>[3x]SVVIVGKISFCPKDVLGHGAEGTIVYRGMFDNRDVAVKRILPECFSFADREVQLLRESDEHPNVIRYFCTEKDRQFQYIAIELCAATLQEYVEQKDFAHLGLEPITLLQQTTSGLAHLHSLNIVHRDLKPHNILISMPNAHG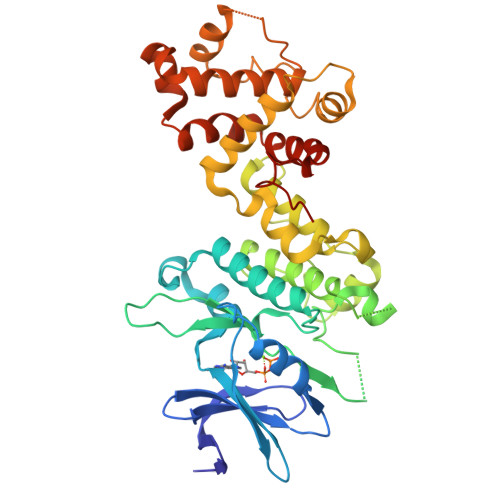KIKAMISDFGLCKKLAVGRHSFSRRSGVPGTEGWIAPEMLSEDCKENPTYTVDIFSAGCVFYYVISEGSHPFGKSLQRQANILLGACSLDCLHPEKHEDVIARELIEKMIAMDPQKRPSAKHVLKHPFFWSLEKQLQFFQDVSDRIEKESLDGPIVKQLERGGRAVVKMDWRENITVPLQTDLRKFRTYKGGSVRDLLRAMRNKKHHYRELPAEVRETLGSLPDDFVCYFTSRFPHLLAHTYRAMELCSHERLFQPYYFHEPP> GSMTSKIALFDQTLIASLLQPLSLNQPDFKAYKTKVKLKISE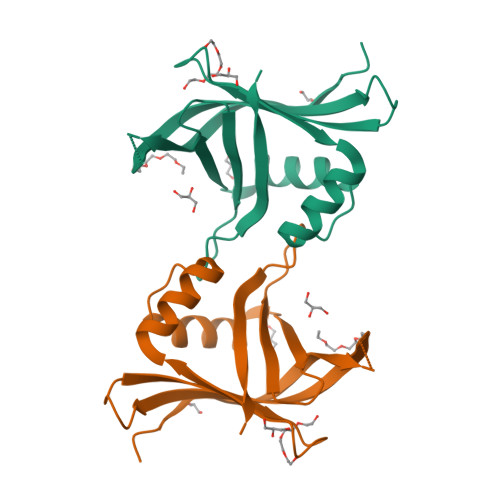QRNETSGEKELKFEISRSDDFEFLFSETLNNEKYQILARDHDLTVDFDAFPKVIIQHLLCKNTEINIILDAEKNFCSFELFSKTPISKGKIFSIKLHAVR Most bacteria proliferate through binary fission, which occurs by the ingrowth of the cell membrane and the peptidoglycan (PG) cell wall to form a septum at midcell. FtsW belongs to the shape, elongation, division, and sporulation (SEDS) family, which functions in cognate pairs with type B penicillin-binding protein (bPBP) family transpeptidases for PG synthesis. The septal PG synthesis is a key step in cell division. As PG synthesis is the primary antibiotic target, Fts complex holds significant antimicrobial potential.

However, the mechanism by which FtsWI is activated is not fully understood. Here, we determined a cryo-EM structure of FtsWI bound to the regulatory proteins FtsQLB at 3.3 Å and performed mutagenic studies to reveal the molecular details for understanding the mechanism of divisome activation. The FtsWIQLB complex from Pseudomonas aeruginosa was expressed, purified, and visualized by a cryo-electron microscope (cryo-EM). The high-resolution cryo-EM map allowed unambiguous assignments for the FtsWIQLB complex, except for FtsQ, of which only the C-terminal β ectodomain (FtsQβ) was resolved. FtsB and FtsL form a long α-helical coiled-coil at the center of the structure, with its N-terminus associated with the transmembrane (TM) α-helical bundle of FtsW, and its C-terminus extending into the periplasmic space, where it interacts with FtsQ and FtsI through their ectodomains. FtsI contains an N-terminal single TM segment (FtsITM) that interacts with FtsW in the TM region and a ‘trophy-like’ C-terminal structure composed of a transpeptidase (TP) domain and a pedestal domain (FtsITP-pedestal), interacting with the FtsBL coiled coil in the periplasm. FtsW comprises ten TM α-helices (TM1–TM10) and a large extracellular loop. TM9 inserts into the central pocket with an angle, together with TM4, TM6, and TM10 forming an outward-open cavity. In our structure, the h2 loop of FtsW is stabilized by FtsL. Moreover, this stabilized h2 loop also positions the putative catalytic residue D275 to interact with conserved residues in the central cavity of FtsW. The binding of the regulatory complex FtsQLB induces the allosteric changes in both FtsW and FtsI to facilitate their activation, including stabilizing the ECL4 loop of FtsW and positioning FtsITP to the site of PG synthesis.

> MLSVLRPFPSPLLSRHGIDLDFPLLAGCLALLGLGLVMVTSASSEVAAAQSGNPLYFSVRHLIYLVIGLISCGLTMMVPMATWQRWGWKLLLVAFGLLVLVITPGIGREVNGSMRWIGFGLFNIQPSEIAKVCVVIFMAGYLIRRQQEVRESWMGFFKPFVVLLPMAGLLLREPDFGATVVMMGAAAAMLFLGGVGLFRFGLMVLLAVGAVVLLIQTQPYRMARLTNFTDPWADQFGAGYQLSQALIAFGRGGWLGMGLGNSIQKQFYLPEAHTDFVFAVLAEELGIVGALATVALFVFVSLRALYIGIWAEQAKQFFSAYVAYGLAFLWIGQFLINIGVNVGLLPTKGLTLPFLSYGGSSLVICCACLGMLLRIEWERRTHLGSEEYEFNEEDFADER;> MKLNYFQGALYPWRFCVIVGLLLAMVGAIVWRIVDLHVIDHDFLKGQGDARSVRHIAIPAHRGLITDRNGEPLAVSTPVTTLWANPKELMTAKERWPQLAAALGQDTKLFADRIEQNAEREFIYLVRGLTPEQGEGVIALKVPGVYSIEEFRRFYPAGEVVAHAVGFTDVDDRGREGIELAFDEWLAGVPGKRQVLKDRRGRVIKDVQVTKNAKPGKTLALSIDLRLQYLAHRELRNALLENGAKAGSLVIMDVKTGEILAMTNQPTYNPNNRRNLQPAAMRNRAMIDVFEPGSTVKPFSMSAALASGRWKPSDIVDVYPGTLQIGRYTIRDVSRNSRQLDLTGILIKSSNVGISKIAFDIGAESIYSVMQQVGLGQDTGLGFPGERVGNLPNHRKWPKAETATLAYGYGLSVTAIQLAHAYAALANDGKSVPLSMTRVDRVPDGVQVISPEVASTVQGMLQQVVEAQGGVFRAQVPGYHAAGKSGTARKVSVGTKGYRENAYRSLFAGFAPATDPRIAMVVVIDEPSKAGYFGGLVSAPVFSKVMAGALRLMNVPPDNLPTATEQQQVNAAPAKGGRG;> MSRLFVKRLPTGSFLMLLLYIGLLLSAIAVAYSTYWNRQLLNSLYSELSVRDKAQAEWGRLILEQSTWTAHSRIESLAVEQLRMRVPDPAEVRMVAP;> MRLRSPYWLFVVLILALAGLQYRLWVGDGSLAQVRDLQKQIADQHGENERLLERNRILEAEVAELKKGTETVEERARHELGMVKDGETLYQLAK;> MNGVLLRHQQPGGLGRAPRKPMPRGASRLVAKEPLSVRLPKADFSFLKYLAWPLLLAVLGYGAYRGAEYILPYADRPIAKVSVEGDLSYISQRAVQQRISPYLAASFFTIDLAGMRGQLEQMPWIAHAEVRRVWPDQVVIRLDEQLPIARWGDEALLNNQGQAFTPKELANYEHLPRLHGPQRAQQQVMQQYQLLSQLLRPLGFSIARLEMSDRGGWALTTAQGVEIQIGRDHVVDKIRRFVSIYDKALKDQISNIARIDLRYPNGLAVAWREPVTPATVATASAVQ> MNNNKIVIMFIFSA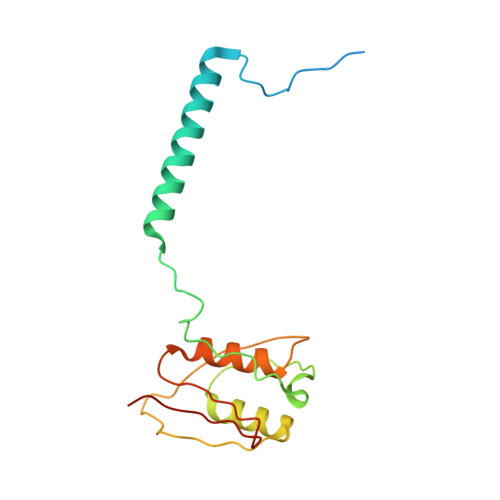LLAGCAGTMKFKKPPINNPSDDATIKLAEAAVSVSDSMLEMAKVEKVITPPSKDNTLTIPNAYNLQARASVDWSGPIEELTARIAKAAHFRFRVLGKSPSVPVLISISTKDESLAEILRDIDYQAGKKASIHVYPNSQVVELRYAKIYS Only a few parasite proteins are exposed on host cell surfaces, and these have mostly diversified into large protein families, allowing a population survival strategy based on antigenic variation. More ubiquitous across Plasmodium species are families of small variant surface antigens (VSAs). These include the CIRs of Plasmodium chabaudi and the VIRs of Plasmodium vivax, often known as the “Plasmodium-interspersed repeats” (PIRs). To determine the structure of a member of the PIR family, we focused on proteins from P. chabaudi, often known as CIRs. These consist of an N-terminal extracellular domain ranging in size from 28 kDa (236 residues) to 133 kDa (1,331 residues) in the AS strain.

Crystals formed for PCHAS_1200500 and contained three copies in the asymmetric unit. A complete dataset was collected to 2.15 Å, and the structure was determined by Sulfur-SAD phasing, using anomalous scattering from the sulfur atoms found in the five disulfide bonds and six methionine residues in each monomer. A complete model was built for residues 5 to 242. Another 20 residues, which connect the ectodomain to the predicted transmembrane helix, are missing from the C terminus, suggesting that this domain is connected to the membrane through a flexible, disordered linker. The CIR ectodomain adopts a compact α-helical structure, arranged into two distinct clusters of helices. The N-terminal half of the ectodomain is formed from five tightly packed helices connected by long loops largely lacking in secondary structure. This packs against the C-terminal portion of the ectodomain, which is folded as a cluster of three parallel helices, connected by short loops. Five disulfide bonds stabilize the fold, supporting the hypothesis that the CIRs are surface proteins, because disulfide bonds are characteristic of proteins located in the oxidizing extracellular environment. The surface opposite this attachment site is dominated by a long loop that links helices 1 and 2. This is one of the most flexible regions of the domain, containing the residues with the highest crystallographic B factors.

>[3x]MENSADNLKYVCKDIKKIDDCLQIDTIYTGVCSDDTLYSDYCPMKNGKKGQCETNNDKISAGFIWLLVMFEHICDDDECSQNEKDQYAGYAILWLSYILNQMPNEGIHTLKNFYTNHIETNTNYASHVSSASDSNYKGIVDKKIDLMNMNKAIIPKFYDIFKSLCNMYNELDKNEANYANCLKDAQNFVDEYQKFLNDNNVDTDDSSYKQILPILSNGYDNLIKKCNNGQHSNFPPLPTTKTTQLSAHISEDTSSSSSIASKLIPTLLIFAIPVFLGIAYKYSLFGFDKRFRRKYSREKLKNKE[(3S)-9-hydroxy-1-methyl-10-oxo-4,10-dihydro-3H-benzo[g]isochromen-3-yl]acetic 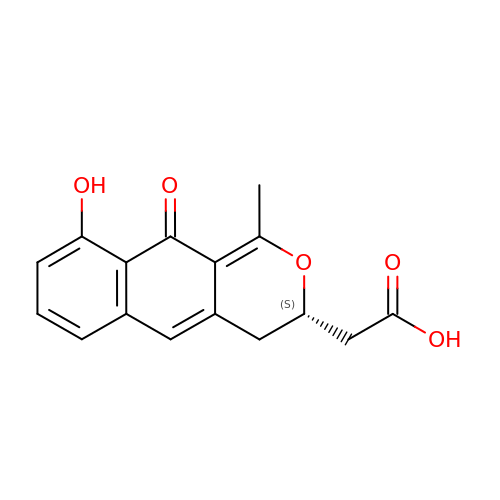acid | C16 H14 O5 | HHXSOTFPYPQSBU-NSHDSACASA-N3,6-Bis[3-(4-methylpiperidino)propionamido]acridine | C31 H41 N5 O2 | 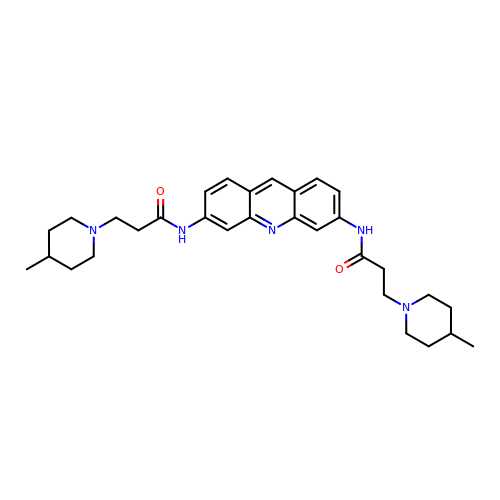BQDBDQOPOGFTHF-UHFFFAOYSA-N> GPHMGGSMFSWLKKGGARGQRPEAIRTVTSSLKELYRTKLLPLEEHYRFGSFHSPALEDADFDGKPMVLVAGQYSTGKTSFIQYLLEQEVPGSRVGPEPTTDCFVAVMHGETEGTVPGNALVVDPEKPFRKLNPFGNTFLNRFMCAQLPNQVLESISIIDTPGILSGAKQRVSRGYD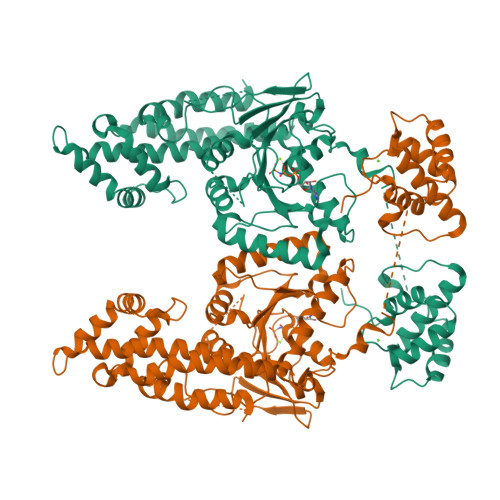FPAVLRWFAERVDLIILLFDAHKLEISDEFSEAIGALRGHEDKIRVVLNKADMVETQQLMRVYGALMWALGKVVGTPEVLRVYIGSFWSQPLLVPDNRRLFELEEQDLFRDIQGLPRHAALRKLNDLVKRARLVRVHAYIISYLKKEMPTVFGKENKKKQLILKLPVIFAKIQLEHHISPGDFPDCQKMQELLMAHDFTKFHSLKPKLLEALDDMLAQDIAKLMPLLRQEELESVEAGVAGGAFEGTRMGPFVERGPDEAIEDGEEGSEDDAEWVVTKDKSKYDEIFYNLAPADGKLSGSKAKTWMVGTKLPNSVLGRIWKLSDVDRDGMLDDEEFALASHLIEAKLEGHGLPTNLPRRLVPPSKRRQKGSAE> MQLTPREVEKLMIYTLSDVAFKRKARGLKLNYPEAVSIITV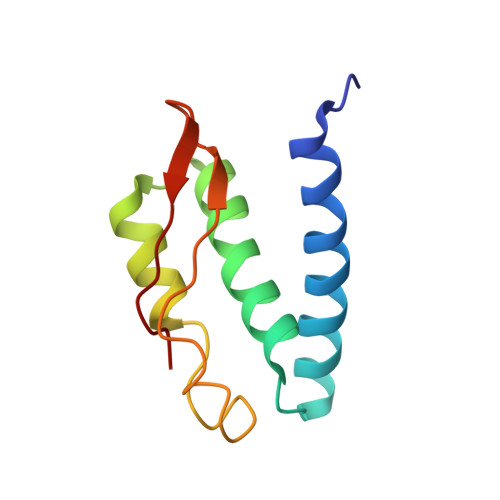TAMEGARDGKSVEDVMKEASKVLTKDDVMDGVADLIPNVQVEAIFTDGSRLVTVHDPIK> EATLGSGNLRQAVMLPEGEDLNEWIAVNTVDFFNQINMLYGTITEFCTEASCPVMSAGPRYEYHWADGTNIKKPIKCSAPKYIDYLMTWVQDQLDDETLFPSKIGVPFPKNFMSVAKTILKRLFRVYAHIYHQHFDSVMQLQEEAHLN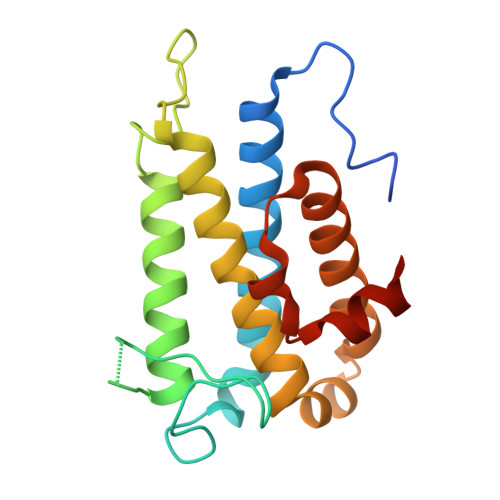TSFKHFIFFVQEFNLIDRRELAPLQELIEKLGSKDR> SKLDLNALNELPKVDRILALAETNAELEKLDAEGRVAWALDNLPGEYVLSSSFGIQAAVSLHLVNQIRPDIPVILTDTGYLFPETYRFIDELTDKLKLNLKVYRATESAAWQEARYGKLWEQGVEGIEKYNDINKVEPMNRALKELNAQTWFAGLRREQSGSRAN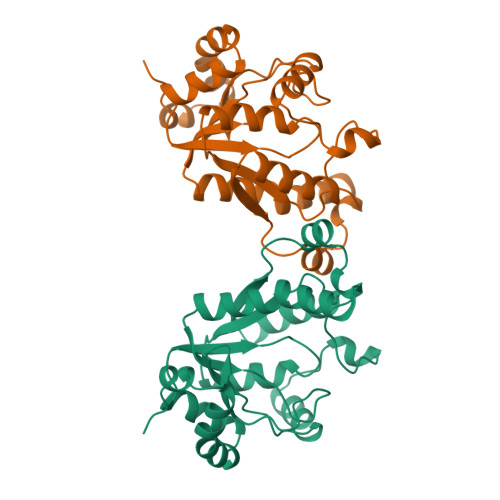LPVLAIQRGVFKVLPIIDWDNRTIYQYLQKHGLKYHPLWDEGYLSVGDTH>SQSTRKKSRRNKWHFGVRCRGDAPEILLAVYRALQRAGAQFTVPKPVNGKYRSDMYTIKSRWEIPHCKREGKNTYAYIELQLYEVMPGCFMLDVKSNGYKDIYSHPERTADHGMDDLKSSFPFLDLCAMLVCKLFSA[2x];>[2x]MSESEQYSTEIPAFLTSNTLQELKLPKPPSLPPHLEKCILNSNTAYKEDQSVLPNPNHVLLNHLAAANTQLGVLALSATTRYHRKYVTTAMFKNFDV;>[2x]AMDVQETQKGALKEIQAFIRSRTSYDVLPTSFRLIVFDVTLFVKTSLSLLTLNNIVSAPLWDSEANKFAGLLTMADFVNVIKYYYQSSSFPEAIAEIDKFRLLGLREVERKIGAIPPETIYVHPMHSLMDACLAMSKSRARRIPLIDVDGETGSEMIVSVLTQYRILKFISMNCKETAMLRVPLNQMTIGTWSNLATASMETKVYDVIKMLAEKNISAVPIVNSE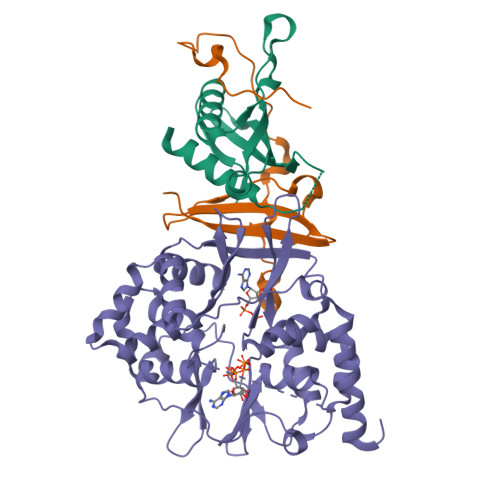GTLLNVYESVDVMHLIQDGDYSNLDLSVGEALLKRPANFDGVHTCRATDRLDGIFDAIKHSRVHRLFVVDENLKLEGILSLADILNYIIYDKTTTPGVPEQTDNFESAV> MEPLYDKNGAVLFGEPSDTHPQSTLKLPHPRGEKEVIVGIRDLPRKGDCRTGNRLGPVSGLFVKPGPVFYQDYSGPVYHRAPLEQFKQAPMCEVTKRIGRVTGSDGNLYHMYVCTDGCILVKTAKREGQDVLKWVYNVLDSPIWVTSC

Npro is a key effector protein of pestiviruses such as bovine viral diarrhea virus and abolishes host cell antiviral defense mechanisms. The nonstructural protein Npro (N-terminal protease) is the very first protein to be synthesized, releasing itself from the nascent polypeptide chain via a single, autoproteolytic cleavage event (Wiskerchen et al., 1991). Detached Npro is proteolytically inactive but acts as a viral immediate effector to modulate the host cell’s antiviral defenses (Ruggli et al., 2003). The overall structure revealed two compacted folding units: a protease domain (orange) and an interaction domain (I-domain, green).

It lacks 21 N-terminal amino acids and carries a C-terminal hexahistidine tag extension for purification purposes (Achmüller et al., 2007). This tag was autoproteolytically removed following in vitro folding from inclusion bodies (IBs), resulting in autoprocessed Δ(2–21)Npro. To elucidate the detailed mechanism of the single autoproteolytic cleavage, we determined the structures of Δ(2–21)Npro and Δ(2–21)Npro S169P6His to 1.5 Å and 2.0 Å resolution, respectively. A product-like conformation resulting from cleavage further delineates Npro’s proteolytic reaction mechanism, revealing three distinct structural elements in catalysis. Consistent with its proposed role as nucleophile in catalysis, we found the first catalytic element Cys69 to be located close to the scissile peptide bond on a distorted α helix. Intriguingly, Cys69 was locked in a disulfide with the P1-residue Cys168, reflecting a ∼3 Å displacement of the Sγ from the position where it could attack the scissile peptide bond. Rather, His49 polarizes the scissile peptide bond carbonyl oxygen through hydrogen bonding and thus supports formation of the tetrahedral transition state intermediate. We determined 1.25 Å and 1.5 Å crystal structures for solubly expressed and in-vitro-folded Npro, respectively. In neither case could we observe zinc binding at the TRASH motif but disulfide bridging between Cys112 and Cys134.3-HYDROXY-2-[(3-HYDROXY-2-METHYL-5-PHOSPHONOOXYMETHYL-PYRIDIN-4-YLMETHYL)-AMINO]-BUTYRIC 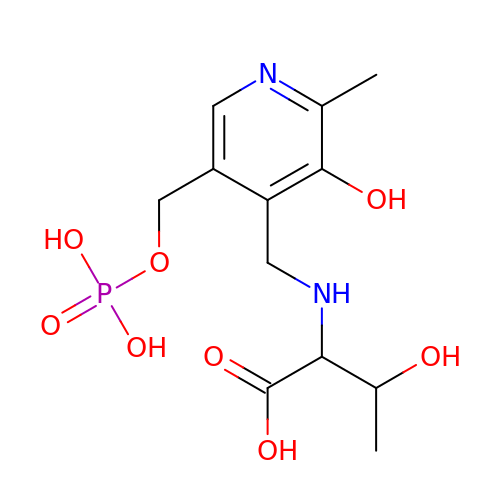ACID | C12 H19 N2 O8 P | IZWQBQLGLAKRMN-UHFFFAOYSA-N> MPAATVDHSQRICEVWACNLDEEMKKIRQVIRKYNYVAMDTEFPGVVARPIGEFRSNADYQYQLLRCNVDLLKIIQLGLTFMNEQGEYPPGTSTWQFNFKFNLTEDMYAQDSIELLTTSGIQFKKHEEEGIETQYFAELLMTSGVVLCEGVKWLSFHSGYDFGYLIKILTNSNLPEEELDFFEILRLFFPVIYDVKYLMKSCKNLKGGLQEVAEQLELERIGPQHQAGSDSLLTGMAFFKMR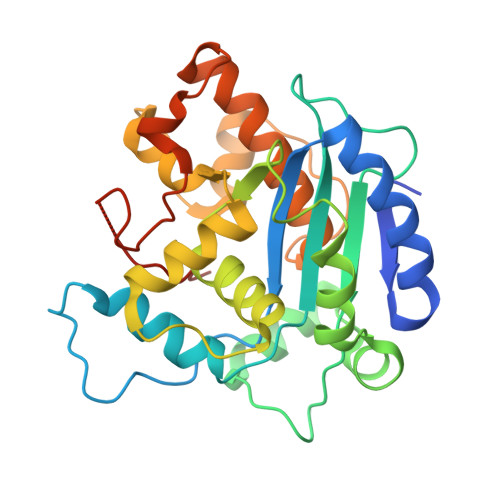EMFFEDHIDDAKYCGHLYGLGSGSSYVQNGTGNAYEEEANKQS> GAACGACACTGA;> CGGGGACTC;> TCACCG;> TCGA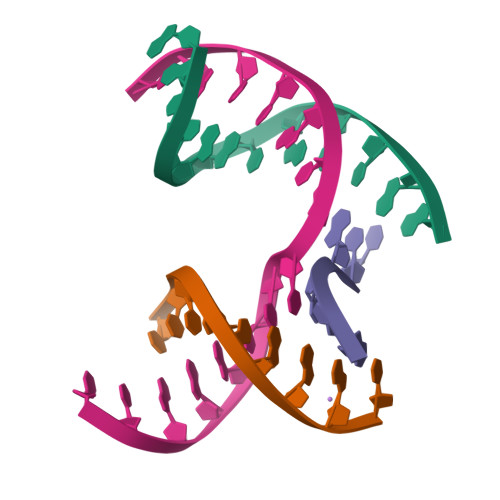GTCCGTGTCGT> AEAGITGTWYNQLGST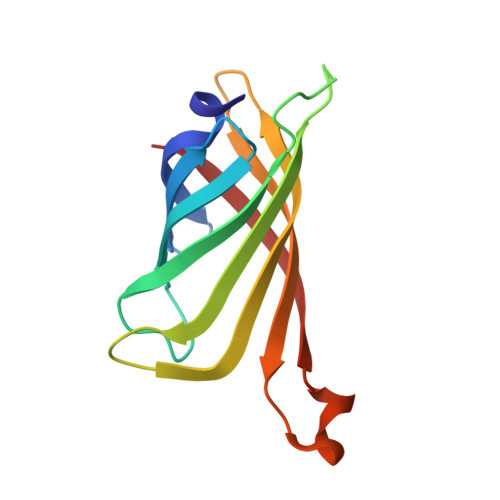FIVTAGADGALTGTYESAVGNAESRYVLTGRYDSAPATDGSGTALGWTVAWKNNYRNAHSATTWSGQYVGGAEARINTQWLLTSGTTEANAWKSTLVGHDTFTKV>MVKVFLVDDHEVVRRGLVDLLGADPELDVVGEAGSVAEAMARVPAARPDVAVLDVRLPDGNGIELCRDLLSRMPDLRCLILTSYTSDEAMLDAILAGASGYVVKDIKGMELARAVKDVGAGRSLLDNRAAAALMAKLRGAAEKQDPLSGLTDQERTLLGLLSEGLTNKQIADRMFLAEKTVKNYVSRLLAKLGM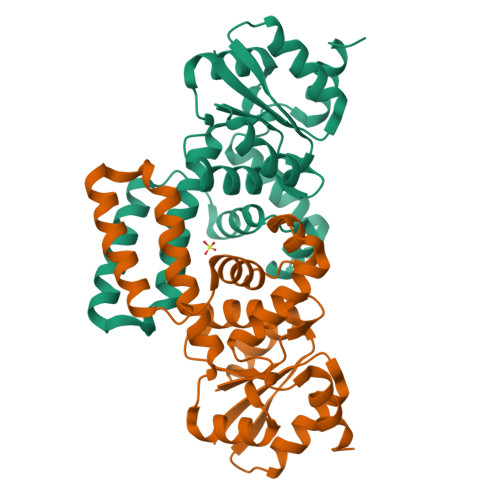ERRTQAAVFATELKRSRPPGDGPLEHHHHHH[2x]> MPDYSYRPTIGRTYVYDNKYYKNLGAVIKNAKRKKHFAEHEIEEATLDPLDNYLVAEDPFLGPGKNQKLTLFKEIRNVKPDTMKLVVGWKGKEFYRETWTRFMEDSFPIVNDQEVMDVFLVVNMRPTRPNRCYKFLAQHALRCDPDYVPHDVIRIVEPSWVGSNNEYRISLAKKGGGCPIMNLHSEYTNSFEQFIDRVIW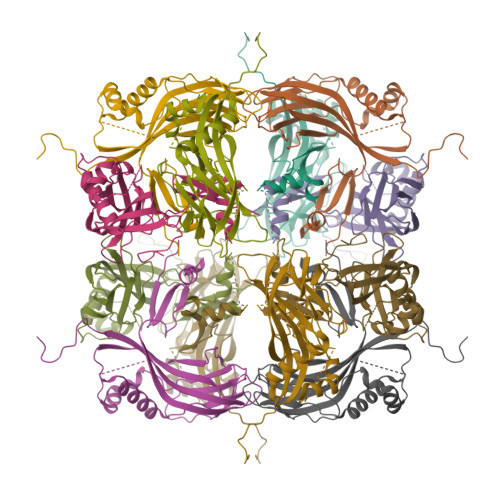ENFYKPIVYIGTDSAEEEEILLEVSLVFKVKEFAPDAPLFTGPAY> IEEGKIVFAVGGAPNEIEYWKGVIAEFEKKYPGVTV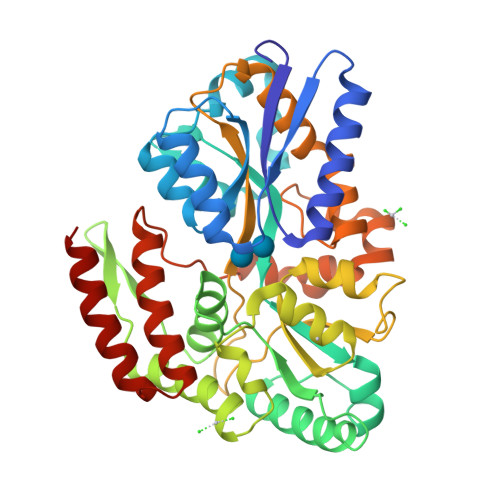ELKRQATDTEQRRLDLVNALRGKSSDPDVFLMDVAWLGQFIASGWLEPLDDYVQKDNYDLSVFFQSVINLADKQGGKLYALPVYIDAGLLYYRKDLLEKYGYSKPPETWQELVEMAQKIQSGERETNPNFWGFVWQGKQYEGLVCDFVEYVYSNGGSLGEFKDGKWVPTLNKPENVEALQFMVDLIHKYKISPPNTYTEMTEEPVRLMFQQGNAAFERNWPYAWGLHNADDSPVKGKVGVAPLPHFPGHKSAATLGGWHIGISKYSDNKALAWEFVKFVESYSVQKGFAMNLGWNPGRVDVYDDPAVVSKSPHLKELRAVFENAVPRPIVPYYPQLSEIIQKYVNSALAGKISPQEALDKAQKEAEELVKQYS>[2x]GAMSEAFHTHSGIGVPLRRSNVDTDQIIP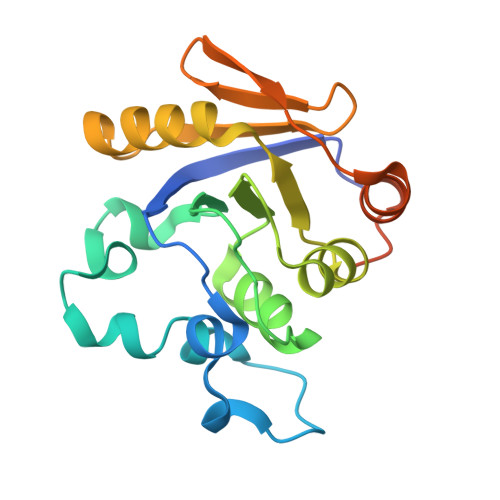AVFLKRVTRTGFEDGLFAGWRSDPAFVLNLSPFDRGSVLVAGPDFGTGSSREHAVWALMDYGFRVVISSRFGDIFRGNAGKAGLLAAEVAQDDVELLWKLIEQSPGLEITANLQDRIITAATVVLPFKIDDHSAWRLLEGLDDIALTLRKLDEIEAFEGA> MEPLYDKNGAVLFGEPSDTHPQSTLKLPHPRGEKEVIVGIRDLPRKGDCRTGNRLGPVSGLFVKPGPVFYQDYSGPVYHRAPLEQFKQAPMCEVTKRIGRVTGSDGNLYHMYVCTDGCILVKTAKREGQDVLKWVYNVLDSPIWVTSCPVDKLAAALEHHHHHH

Npro is a key effector protein of pestiviruses such as bovine viral diarrhea virus and abolishes host cell antiviral defense mechanisms. The nonstructural protein Npro (N-terminal protease) is the very first protein to be synthesized, releasing itself from the nascent polypeptide chain via a single, autoproteolytic cleavage event (Wiskerchen et al., 1991). Detached Npro is proteolytically inactive but acts as a viral immediate effector to modulate the host cell’s antiviral defenses (Ruggli et al., 2003). The overall structure revealed two compacted folding units: a protease domain (orange) and an interaction domain (I-domain, green).

In order to compare this postcleavage, product-like Npro with a precleavage, substrate-like variant, we produced an S169P mutant Δ(2–21)Npro S169P6His, as proline in P1′ was shown to prevent autoproteolysis (Achmüller et al., 2007). To elucidate the detailed mechanism of the single autoproteolytic cleavage, we determined the structures of Δ(2–21)Npro and Δ(2–21)Npro S169P6His to 1.5 Å and 2.0 Å resolution, respectively. We provide mechanistic insight into the proteolytic assembly by describing a substrate-like, unprocessed P1′-site reaction intermediate. Here, a solvent molecule trapped at the active site offers a consistent reaction mechanism highlighting distinct roles of the catalytic water. First, the solvent molecule reveals an untypically short bond distance to the Gly67 amide of 2.3 Å, indicative of a short strong hydrogen bond (SSHB, aka low-barrier hydrogen bond) typically ranging from 2.3 Å to 2.5 Å. Third, the positively charged side chains of Arg70 and Lys66 contribute to stabilize the hydroxide within the anion binding site. Several indications point to the existence of a hydroxide ion at the anion binding site. The geometric proximity of the activated water molecule to the scissile peptide bond suggests its relevance in catalysis. The substrate strand β4 with its P6–P1 residues is rigidly anchored to the edge strand β2 and His49 by a hydrogen bond network both before and after cleavage.> MASHLASIYGTEQDKVNCSFYYKIGACRHGERCSRKHVKPNFSQTILCPNMYKNPIHEPNGKKFTQRELAEQFDAFYEDMFCEFSKYGEVEQLVVCDNVGDH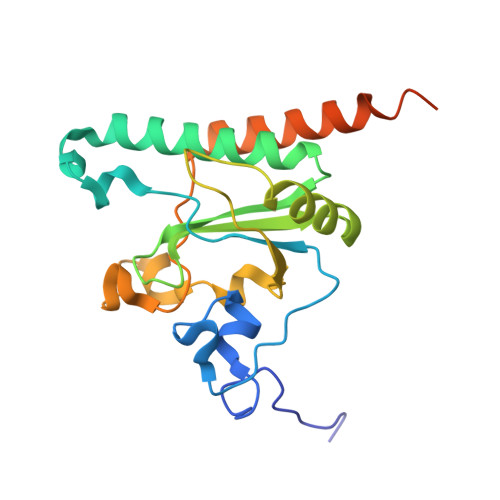LVGNVYVRFKYEESAQNAIDDLNSRWYSQRPVYAELSPVTDFREACCRQHETSECQRGGLCNFMHAKKPSPQLLRDLVLAQRKYLALNAAEEMKKEPNSDSTNRWVSVTAERKN>MRFIHALLLAGIAHSAYASEKLTFKTDLEKLEREKAAQIGVAIVDPQGEIVAG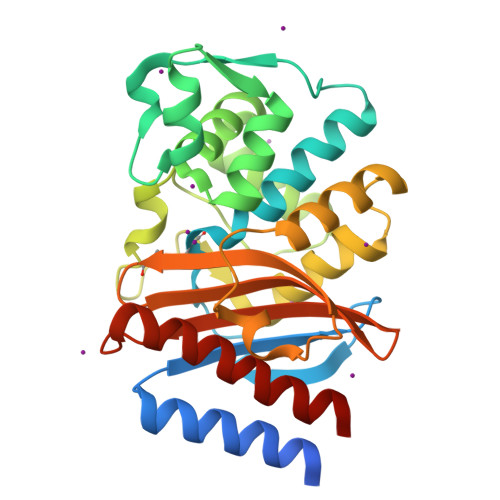HRMAQRFAMCSTFKFPLAALVFERIDSGTERGDRKLSYGPDMIVEWSPATERFLASGHMTVLEAAQAAVQLSDNGATNLLLREIGGPAAMTQYFRKIGDSVSRLDRKEPEMGDNTPGDLRDTTTPIAMARTVAKVLYGGALTSTSTHTIERWLIGNQTGDATLRAGFPKDWVVGEKTGTCANGARNDIGFFKAQERDYAVAVYTTAPKLSAVERDELVASVGQVITQLILSTDK[2x]AMDHD2 is an amidohydrolase that plays a potential role in the HBP by catalyzing the deacetylation of GlcNAc-6P in the ‘reverse’ direction of the pathway. Human AMDHD2 is organized into two domains, a deacetylase domain responsible for the conversion of GlcNAc-6P into GlcN6P and a second small domain with unknown function (DUF). The structure of the deacetylase domain showed a TIM (triosephosphate isomerase) barrel-like fold. In summary, our data show that human AMDHD2 is an obligate dimeric protein with high specificity for GlcNAc-6P that carries a single catalytic Zn ion in the active center.

Optimized crystals diffracted to a resolution limit of 1.84 Å (AMDHD2+Zn) or 1.90 Å (AMDHD2+Zn+GlcN6P). A superposition of the Zn-bound and the GlcN6P- and Zn-bound structures of AMDHD2 indicated no structural changes by the binding of the product. Residues from both monomers contribute to GlcN6P-binding. The phosphate group of the sugar is interacting via hydrogen bonds with Asn235 and Ala236, as well as ionic interactions to His242* and Arg243* of the other monomer. GlcN6P binding to the active site is further mediated by hydrogen bonds between the hydroxyl groups of GlcN6P with Ala154 and His272. The catalytic Zn ion is coordinated via electrostatic interactions with Glu143, His211, His232, and two water molecules, which in turn are stabilized by interactions with GlcN6P and several amino acid side chains including Asp294 that might, based on the homology to bacterial NagA, act as the catalytic base (Hall et al., 2007). Residues from both monomers contribute to ligand binding in the active site, while the residues important for catalysis originate from one monomer. To assess a functional role of the residues His242* and Arg243*, and especially of the dimeric state on catalytic activity of AMDHD2, we generated the double mutant H242A/R243A and the mutants I280E and I280R, whose side chains might disrupt dimerization. Strikingly, I280E, I280R, andH242A/R243A showed no catalytic activity, supporting that AMDHD2 must form a dimer to be active and that the residues His242* and Arg243* are indispensable for catalytic activity.

>MRGEQGAAGARVLQFTNCRILRGGKLLREDLWVRGGRILDPEKLFFEERRVADERRDCGGRILAPGFIDVQINGGFGVDFSQATEDVGSGVALVARRILSHGVTSFCPTLVTSPPEVYHKVVPQIPVKSGGPHGAGVLGLHLEGPFISREKRGAHPEAHLRSFEADAFQDLLATYGPLDNVRIVTLAPELGRSHEVIRALTARGICVSLGHSVADLRAAEDAVWSGATFITHLFNAMLPFHHRDPGIVGLLTSDRLPAGRCIFYGMIADGTHTNPAALRIAHRAHPQGLVLVTDAIPALGLGNGRHTLGQQEVEVDGLTAYVAGTKTLSGSIAPMDVCVRHFLQATGCSMESALEAASLHPAQLLGLEKSKGTLDFGADADFVVLDDSLHVQATYISGELVWQADAARQ[2x]2-[(furan-2-ylmethyl)amino]ethanesulfonic 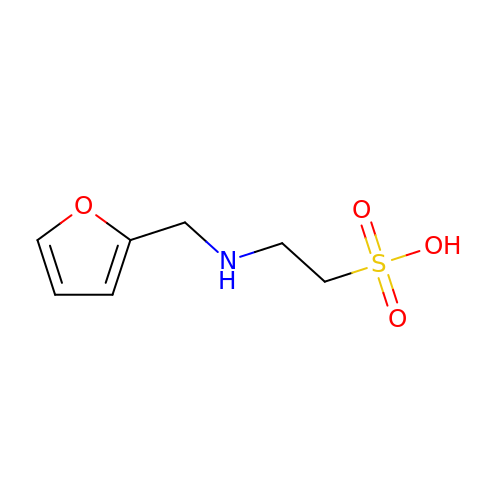acid | C7 H11 N O4 S | HKTRCFGIKAIPHE-UHFFFAOYSA-N> MVDY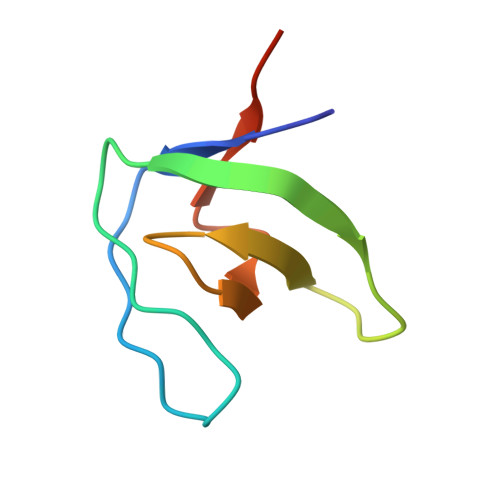IVEYDYDAVHDDELTIRVGEIIRNVKKLQEEGWLEGELNGRRGMFPDNFVKEIKRETE>[2x]PHMSGLKKFFPYSTNVLKGAAADIALPSLAGKTVFFYFSASWCPPCRAFTPQLIDFYKAHAEKKNFEVMLISWDESAEDFKDYYAKMPWLALPFEDRKGMEFLTTGFDVKS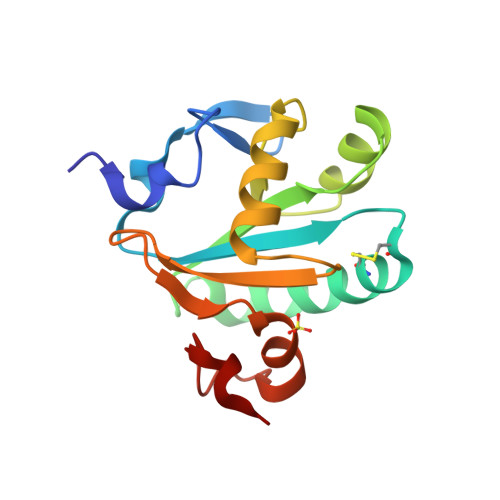IPTLVGVEADSGNIITTQARTMVVKDPEAKDFPWPNVEAKK~{N}-methyl-3-(3-methylbutyl)-5-oxidanyl-1,2,3-triazole-4-carboxamide 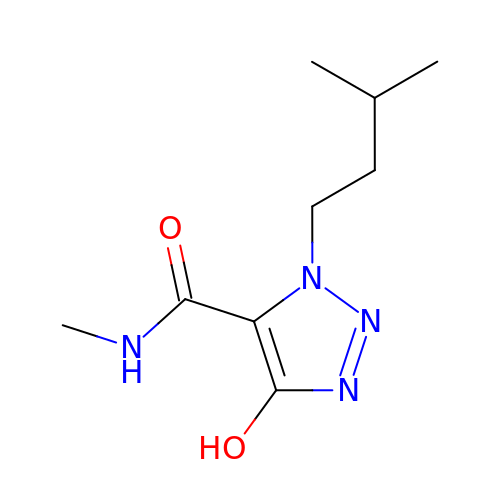| C9 H16 N4 O2 | DKBFJEZTUMLWCW-UHFFFAOYSA-N> GAQVSRQQTGTHENANVATGGSSITYNQINFYKDSYAASASKQDFSQDPSKFTEPVAEALKA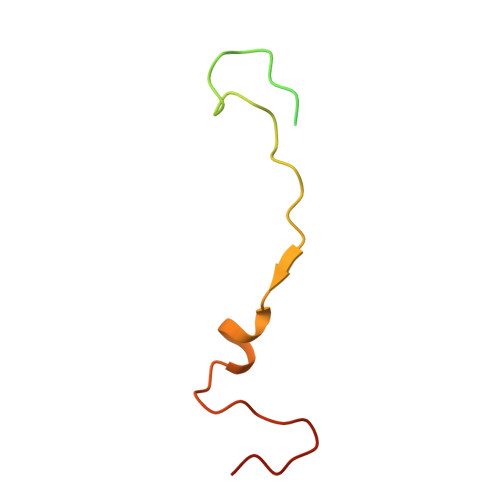GAPVLK>MPAVTQPRGESKYDAIPGPLGPQSASLEGKVALVTGAGRGIGREMAMELGRRGCKVIVNYANSTESAEEVVAAIKKNGSDAACVKANVGVVEDIVRMFEEAVKIFGKLDIVCSNSGVVSFGHVKDVTPEEFDRVFTINTRGQFFVAREAYKHLEIGGRLILMGSITGQAKAVPKHAVYSGSKGAIETFARCMAIDMADKKITVNVVAPGGIKTDMYHAVCREYIPNGENLSNEEVDEYAAVQWSPLRRVGLPIDIARVVCFLASNDGGWVTGKVIGIDGGA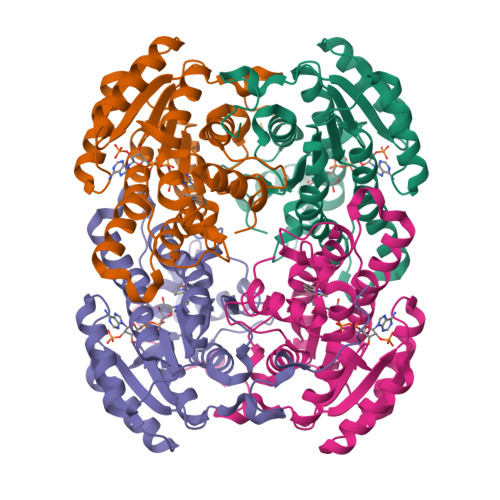CM[4x]> DRSEATLIKRFKGEGVRYKAKLIGIDEVSAARGDKLCQDSMMKLK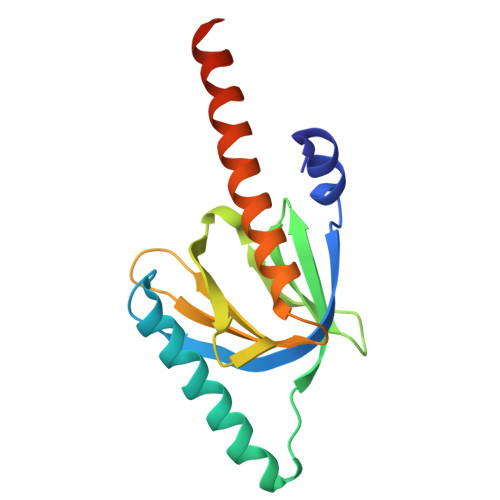GVVAGARSKGEHKQKIFLTISFGGIKIFDEKTGALQHHHAVHEISYIAKDITDHRAFGYVCGKEGNHRFVAIKTAQAAEPVILDLRDLFQLIYELKQREELEKKAQKDKQCEQA Muramidases (N-acetylmuramide glycanhydrolases), also known as lysozymes, cleave the bacterial cell wall peptidoglycan component at the β-1,4-glycosidic bond between N-acetylmuramic acid (NAM) and N-acetylglucosamine (NAG) in the carbohydrate backbone. The characterized enzymes from GH25 exhibit both β-1,4-N-acetyl- and β-1,4-N,6-O-diacetylmuramidase activities, cleaving the β-1,4-glycosidic bond between N-acetylmuramic acid (NAM) and N-acetylglucosamine (NAG) moieties in the carbohydrate backbone of bacterial peptidoglycan. The first half of the barrel, where the active site residues are located, is a classical barrel which is consistent with the idea that the initial ancient fold was a half-barrel which became an eight stranded barrel by gene duplication, with more sequence conservation in the half that contains the catalytic residue and less sequence (and as seen here structure) conservation in the other half which is responsible for binding specific targets. It is proposed that, as previously suggested for other GH25 muramidases, that Asp95 acts as an acid donating a proton to the glycosidic oxygen of the substrate, with the N-acetyl group of the substrate rather than a second protein carboxylate acting as the enzymatic nucleophile to stabilise the oxocarbenium ion-like transition state.

The enzyme from Acremonium alcalophilum JCM 7366 (A. alcalophilum is now known as Sodiomyces alcalophilus (G. Okada) Giraldo López & Crous, but we will use the AaMur abbreviation for the muramidase in this paper) finally proved to be the muramidase of choice. For AaMur, there was a single molecule in the asymmetric unit and the whole chain was modelled, with only the terminal residues Arg1 and Asp208 being rather poorly defined. The catalytic residues in the conserved GH25 DXE motif are Asp95 and Glu97. The density is typical for such a high-resolution structure showing essentially resolved carbon, oxygen and nitrogen atoms, with many of the hydrogen atoms seen in the difference density. A strong H-bond is shown between the catalytic acid Asp95 and its conserved supporting residue Glu97. The high quality of the structure at 0.78Å is evident from the weighted map and in the difference map there are positive density peaks for a good number of the hydrogen atoms. TzMur, Zopfiella sp. t180-6 and Ascobolus stictoideus had Tm above 60°C at both pH 3 and 5. The melting temperature of AaMur as a function of pH using three different buffers is shown in Table 5, establishing that it retained its stability over a range of pH. The optimum is at pH 4.0, but the activity profiles are quite broad, especially for AaMur.

> RIPGFDISGWQPTTDFARAYANGDRFVYIKATEGTTFKSSAFSRQYTGATQNGFIRGAYHFAQPAASSGAAQARYFASNGGGWSKDGITLPGALDIEYNPNGATCYGLSQSAMVNWIEDFVTTYHGITSRWPVIYTTTDWWTQCTGNSNRFANRCPLWIARYASSVGTLPNGWGFYTFWQYNDKYPQGGDSNWFNGDASRLRALANGD>[8x]HMSIITDVYAREVLDSRGNPTLEVEVYTESGAFGRGMVPSGASTGEHEAVELRDGDKSRYLGLGTQKAVDNVNNIIAEAIIGYDVRDQQAIDRAMIALDGTPNKGKLGANAILGVSIAVARAAADYLEVPLYTYLGGFNTKVLPTPMMNIINGGSHSDAPIAFQEFMIMPVGAPTFKEGLRWGAEVFHALKKILKERGLVTAVGDEGGFAPKFEGTEDGVETILKAIEAAGYEAGENGIMIG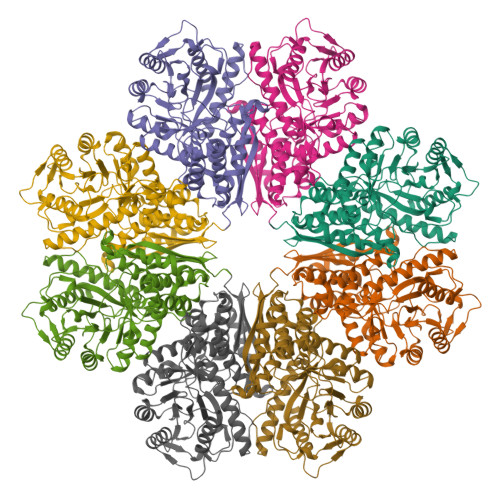FDCASSEFYDKERKVYDYTKFEGEGAAVRTSAEQVDYLEELVNKYPIITIEDGMDENDWDGWKVLTERLGKRVQLVGDDFFVTNTEYLARGIKENAANSILIKVNQIGTLTETFEAIEMAKEAGYTAVVSHRSGETEDSTIADIAVATNAGQIKTGSLSRTDRIAKYNQLLRIEDQLGEVAQYKGIKSFYNLKK>[5x]GQDMVSPPPPIADEPLTVNTGIYLIECYSLDDKAETFKVNAFLSLSWKDRRLAFDPVRSGVRVKTYEPEAIWIPEIRFVNVENARDADVVDISVSPDGTVQYLERFSARVLSPLDFR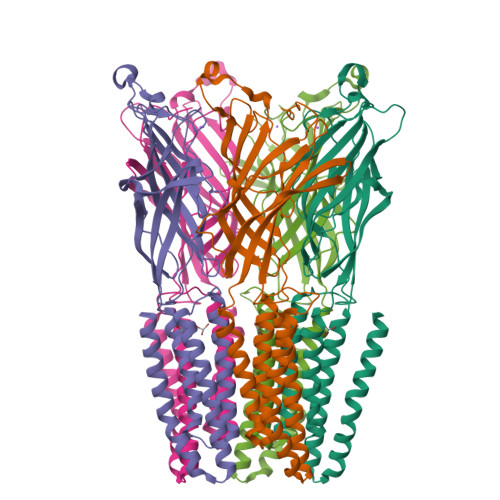RYPFDSQTLHIYLIVRSVDTRNIVLAVDLEKVGKNDDVFLTGWDIESFTAVVKPANFALEDRLESKLDYQLRISRQYFSYIPNIILPMLFILFISWTAFWSTSYEANVTLVVSTLIAHIAFCILVETNLPKTPYMTYTGAIIFMIYLFYFVAVIEVTVQHYLKVESQPARAASITRASRIAFPVVFLLANIILAFLFFGFGYPYDVPDYA>[2x]HHHMSEATLLSYTKKLLASPPQLSSTDLHDALLVILSLLQKCDTNSDESLSIYTKVSSFLTALRVTKLDHKAEYIAEAAKAVLRHSDLVDLPLPKKDELHPEDGPVILDIVGTGGDGQNTFNVSTSA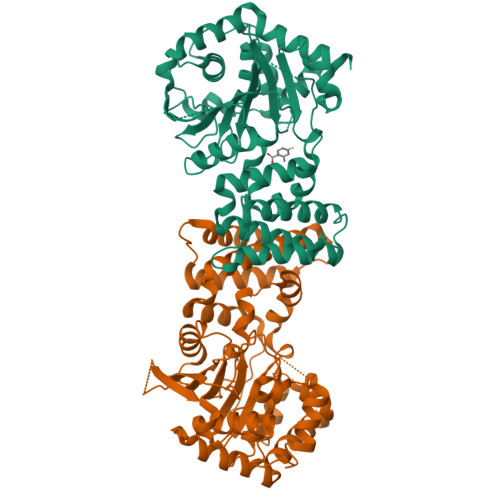AIVASGIQGLKICKHGNKASTSNSGAGDLIGTLGCDMFKVNSSTVPKLWPDNTFMFLLAPFFHHGMGHVSKIRKFLGIPTVFNVLGPLLHPVSHVNKRILGVYSKELAPEYAKAAALVYPGSETFIVWGHVGLDEVSPIGKTTVWHIDPTSSELKLKTFQLEPSMFGLEEHELSKCASYGPKENARILKEEVLSGKYHLGDNNPIYDYILMNTAVLYCLSQGHQNWKEGIIKAEESIHSGNALRSLEHFIDSVSSL>[4x]MTMRYQEPARIPNAEIDHVLASGNPEAIADA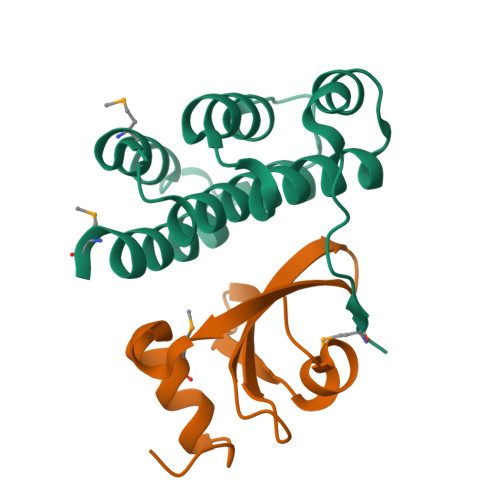CLSIAYYEDDWEWAFKRLKSVAFDLNRPDSLRSLAVTCVGHLARRIHDLDVAMAEEFLLSLGGDQAVASAASDALDDLRIFRMSD;>[4x]SRGPSNGQSVLENSVQVKETSPRRVSVDPQTGEFVVFDRTLGDVYHGHVRAWKDLTSDMQNALVRGGYVDRKGNPK> GPAAGNMNSGIAAFEMEYTHWLEEQNRRVSEIRTALQAHIGDIELKMLVDSCLNHYANLFRMKADAAKADVFFLMSGMWRTSTERFFQWIGGFRPSELLNVVMPYVEPLTDQQLLEVRNLQQSSQQAEEALSQGLDKLQQGLVESIAIQIKVVESVNHGAPMASAMENLQALESFVNQADHLRQQTLQQMSKILTTRQAARGLLALGEYFH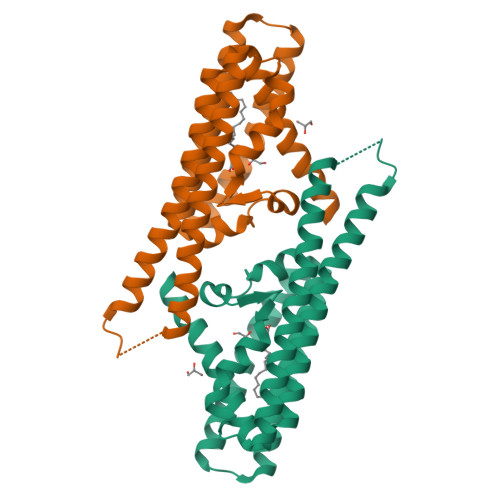RLRALSSLWAARPREHTGGDYKDDDDKSSGYPYDVPDYA>[8x]MRQETRFKFNAYLSRVAELNGIDAGDVSKKFTVEPSVTQTLMNTMQESSDFLTRINIVPVSEMKGEKIGIGVTGSIASTTDTAGGTERQPKDFSKLASNKYECDQINFDFYIRYKTLDLWARYQDFQLRIRNAIIKRQSLDFIMAGFNGVKRAETSDRSSNPMLQDVAVGWLQKYRNEAPARVMSKVTDEEGRTTSEVIRVGKGGDYASLDALVMDATNNLIEPWYQEDPDLVVIVGRQLLADKYFPIVNKEQDNSEMLAADVIISQKRIGNLPAVRVPYFPADAMLITKLENLSIYYMDDSHRRVIEENPKLDRVENYESMNIDYVVEDYAAGCLVEKIKVGDFSTPAKATAEPGA;>[2x]MSDHTIPEYLQPALAQLEKARAAHLENARLMDETVTAIERAEQEKNALAQADGNDADDWRTAFRAAGGVLSDELKQRHIERVARRELVQEYDNLAVVLNFERERLKGACDSTATAYRKAHHHLLSLYAEHELEHALNETCEALVRAMHLSILVQENPLANTTGHQGYVAPEKAVMQQVKSSLEQKIKQMQISLTGEPVLRLTGLSAATLPHMDYEVAGTPAQRKVWQDKIDQQGAELKARGLLS

P2 procapsids are assembled from pentamers and hexamers of the major capsid protein, gpN on a T = 7 dextro icosahedral lattice, together with the internal scaffolding protein, gpO, and a dodecamer of the portal protein (traditionally called “connector”), gpQ, at a single, unique capsid vertex. “Satellite” phage P4 is not a true phage, but rather a “pirate” mobile genetic element (MGE) —an integrative plasmid that has acquired the ability to utilize a “helper” phage, such as P2, for its own propagation. However, the Sid (“Size determination”) protein encoded by P4 changes the P2 capsid from its normal 60 nm diameter, T = 7 organization to a 45 nm capsid with T = 4 architecture. The smaller capsid fits the 11.6 kb P4 genome, but is too small to package the 33.6 kb P2 genome, thereby leading to strong suppression of P2 burst size.

P4 procapsids were generated by E. coli co-expression of gpN, Sid and a protease-deficient form of gpO [O(S107A)], purified on sucrose gradients, and prepared for cryo-EM by standard methods. The remaining particles were refined with an expanded soft mask and without symmetry averaging, resulting in an asymmetric reconstruction of the P4 procapsid at a resolution of 4.19 Å (FSC = 0.143). The P4 procapsid is organized on a T = 4 lattice, resulting in four copies of gpN in the icosahedral asymmetric unit, here denoted by subscripts A–D (and A2–D2 for the second asymmetric unit). The gpNA (green) subunits form the pentamers at the icosahedral fivefold symmetry axes, while two copies each of gpNB (yellow), gpNC (red) and gpND (blue) form the hexamer at the icosahedral twofold axis. gpN has the expected canonical HK97-like phage capsid protein fold, consisting of an N-arm, an E-loop, a P-domain and an A-domain. Sixty copies of Sid form a dodecahedral cage surrounding the P4 procapsid, interacting with the underlying capsid shell only at the hexamers, and forming trimeric connections at the icosahedral threefold axes. Sid is a highly elongated (126 Å), aliform structure, consisting of five extended α-helices interspersed by loops, the longest of which (residues 189–219) contains an additional short helix. Residues 139–189 form an extensive dimerization interface that includes helices α3 and α4, where the two monomers of Sid interlock in a knot-like structure overlaying the two-fold symmetry axis. Each Sid monomer forms two sets of contacts with the procapsid, exclusively interacting with the two gpNB subunits in each hexamer. In this way, each copy of Sid in the dimer binds to both gpNB subunits in a hexamer, forming a bridge that straddles the hexamer. Therefore, Sid must induce the arrangement of hexamers seen in the T = 4 lattice by forming these trimeric interactions, thus redirecting procapsid assembly towards the smaller architecture suitable only for packaging of the P4 genome.>SNHTYRVIEIVGTSPDGVDAAIQG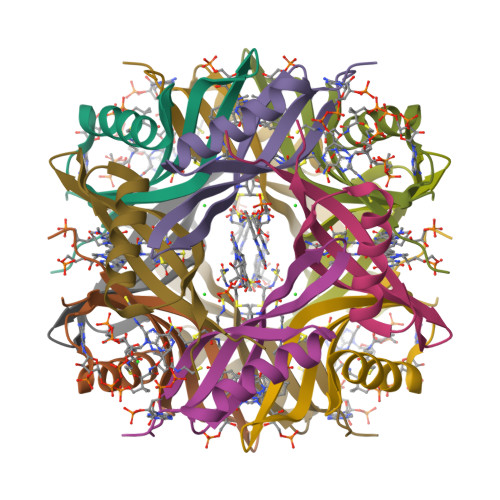GLARAAQTMRALDWFEVQSIRGHLVDGAVAHFQVCMKVGFRLEDS[6x]> PVPTGVSFDYIVVGGGAGGIPAADKLSEAGKSVLLIEKGFASTANTGGTLGPEWLEGHDLTRFDVPGLCNQIWVDSKGIACEDTDQMAGCVLGGGTAVNAGLWFKPYSLDWDYLFPDGWKYNDVQPAINRALSRI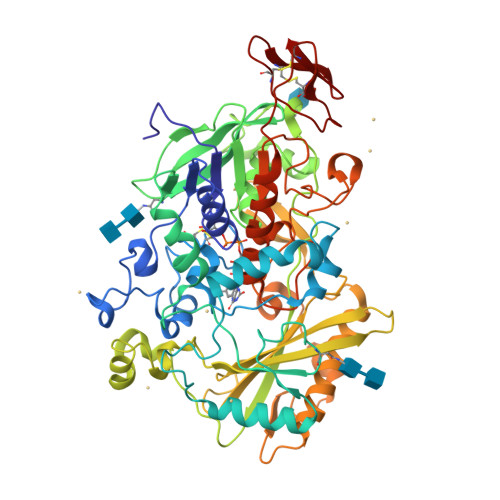PGTDAPSTDGKRYYQEGFEVLSKGLAAGGWTSVTANNAPDKKNRTFAHAPFMFAGGERNGPLGTYFQTAKKRNNFDVWLNTSVKRVIREGGHITGVEVEPFRDGGYEGIVPVTKVTGRVILSAGTFGSAKILLRSGIGPEDQLEVVAASEKDGPTMIGNSSWINLPVGYNLDDHLNTDTVISHPDVVFYDFYEAWDDPIESDKNSYLESRTGILAQAAPNIGPMFWEEIVGADGIVRQLQWTARVEGSLGAPNGHTMTMSQYLGRGATSRGRMTITPSLTTIVSDVPYLKDPNDKEAVIQGIINLQNALQNVANLTWLFPNSTITPREYVESMVVSPSNRRSNHWMGTNKLGTDDGRKGGSAVVDLDTRVYGTDNLFVIDASIFPGVPTTNPTSYIVVAAEHASSRILALPDLEPVPKYGQCGGREWTGSFVCADGSTCEYQNEWYSQCL>[4x]MKGKMAIVISTLNNPWFVVLAETAKQRAEQLGYEATIFDSQNDTAKESAHFDAIIAAGYDAIIFNPTDADGSIANVKRAKEAGIPVFCVDRGINARGLAVAQIYSDTSTQFPKLMA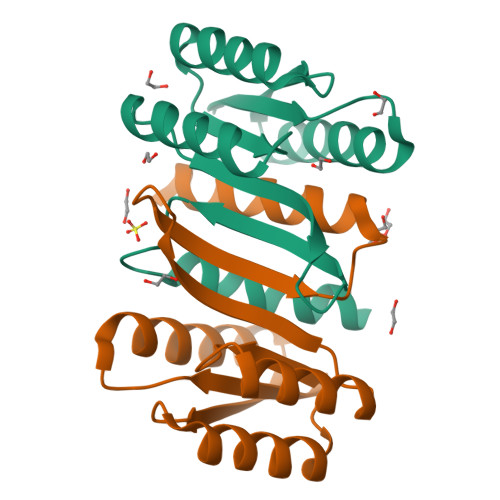RLAVEWADQYLRGGLEHHHHHH>AMTMAKTLKDLQGWEIITTDEQGNIIDGGQKRLRRRGAKTEHYLKRSSDGIKLGRGDSVVMHNEAAGTYSVYMIQELRLNTLNNVVELWALTYLRWFEVNPLAHYRQFNPDANILNRPLNYYNKLFSETANKNELYLTAELAELQLFNFIRVANVMDGSKWEVLKGNVDP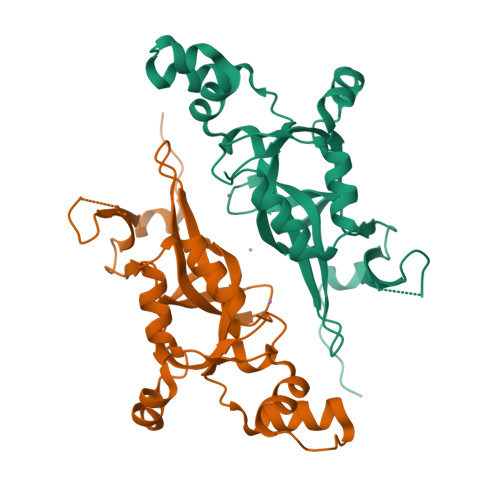ERDFTVRYICEPTGEKFVDINIEDVKAYIKKVEPREAQEYLKDLTLPSKKKEIKRGPQKKDKATQTAQ[2x]>[4x]MSKWTYFGPDGENSWSKKYPSCGGLLQSPIDLHSDILQYDASLTPLEFQGYNLSANKQFLLTNNGHSVKLNLPSDMHIQGLQSRYSATQLHLHWGNPNDPHGSEHTVSGQHFAAELHIVHYNSDLYPDASTASNKSEGLAVLAVLIEMGSFNPSYDKIFSHLQH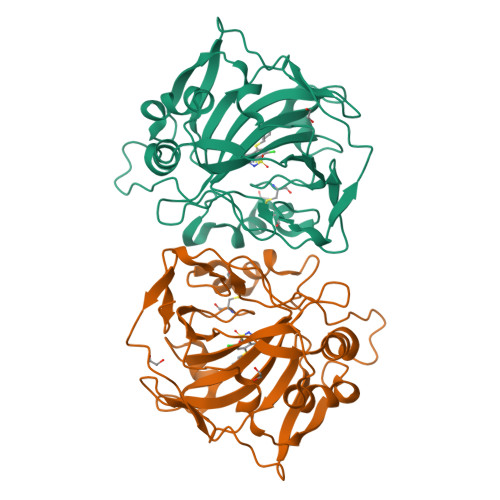VKYKGQEAFVPGFNIEELLPERTAEYYRYRGSLTTPPCNPTVLWTVFRNPVQISQEQLLALETALYCTHMDDPSPREMINNFRQVQKFDERLVYTSFSQ> SAMNNEGKALMAIKGSFSNLVNMLLDWDDVHNSDLCSWRGVFCDNVSYSVVSLNLSSLNLGGEISPAIGDLRNLQSIDLQGNKLAGQIPDEIGNCASLVYLDLSENLLYGDIPFSISKLKQLETLNL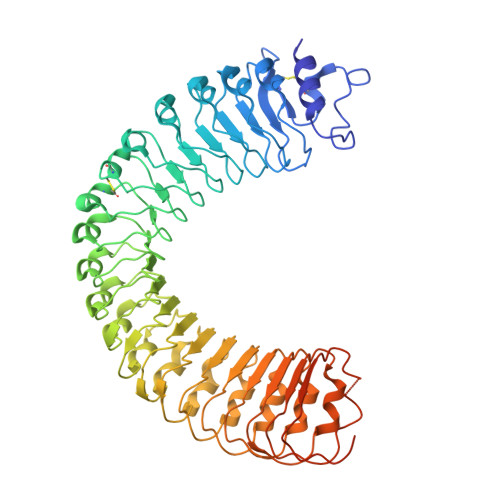KNNQLTGPVPATLTQIPNLKRLDLAGNHLTGEISRLLYWNEVLQYLGLRGNMLTGTLSSDMCQLTGLWYFDVRGNNLTGTIPESIGNCTSFQILDISYNQITGEIPYNIGFLQVATLSLQGNRLTGRIPEVIGLMQALAVLDLSDNELVGPIPPILGNLSFTGKLYLHGNMLTGPIPSELGNMSRLSYLQLNDNKLVGTIPPELGKLEQLFELNLANNRLVGPIPSNISSCAALNQFNVHGNLLSGSIPLAFRNLGSLTYLNLSSNNFKGKIPVELGHIINLDKLDLSGNNFSGSIPLTLGDLEHLLILNLSRNHLSGQLPAEFGNLRSIQMIDVSFNLLSGVIPTELGQLQNLNSLILNNNKLHGKIPDQLTNCFTLVNLNVSFNNLSGIVPPMKNFSRFAPASFVGNPYLCGNWVGSICGHHHHHH>[4x]GPLGSDYIIKEKTVLLQKKDSEGFGFVLRGAKAQTPIEEFTPTPAFPALQYLESVDEGGVAWRAGLRMGDFLIEVNGQNVVKVGHRQVVNMIRQGGNTLMVKVVMVTRHPDM;>[4x]EESTSFQGP

The SHANK (SH3 and multiple ankyrin repeat domain) protein acts as a scaffolding protein located at excitatory glutamatergic synapses; it plays a crucial role in synapse formation, maintenance, function, and development. As one of the key components of SHANK structures, PDZ [Postsynaptic density protein-95(PSD-95)/Discs-large (DLG)/zonula occludens-1(ZO1)] domains are a large class of protein–protein interaction (PPI) modules that are widely conserved from yeast to humans. A canonical PDZ domain is usually composed of roughly 90 amino acid residues, consisting of 5–6 β-strands (βA-βF) capped by a short helix αA and a long α-helix αB, where the N- and C-terminal strands βA and βF are in mutual proximity. Significantly, PDZs possess a highly conserved carboxylate-binding loop formed by the second α-helix (αB) and the second β-strand (βB) in an antiparallel fashion; discoveries and characterization of PBMs have established that C-terminal PBMs predominate.

Here we characterize a short linear motif (SLiM) — EESTSFQGP — as an internal PBM based on its strong binding affinity towards the SHANK1 PDZ domain (SHANK1656–762 hereafter referred to as SHANK1). To obtain further insight into the molecular basis of the SHANK1/Ac-EESTSFQGP-NH2 interaction, the co-crystal structure was solved at a resolution of 1.98 Å. The crystals used for structure determination belonged to the trigonal space group P3221. X-ray crystallographic analyses on the SHANK1/Ac-EESTSFQGP-CONH2 complex identified an asymmetric tetramer with four similar protein-ligand protomers. Overall, the two SHANK1 backbones exhibit extensive overlap with an RSMD of 0.45 Å, with subtle differences within the loops, e.g. Q667-G675PDZ, G680-Q700PDZ, V705-G709PDZ and G748-T748PDZ. Loop flexibility likely contributes to adaptation for binding of the different ligands; comparing the SHANK1/Ac-EESTSFQGP-NH2 and SHANK1/GKAP PBM structures, the loops in the Ac-EESTSFQGP-NH2 bound PDZ appear slightly extended so as to accommodate the N-terminal acetyl group as well as the C-terminal extended motif [Gln (1) — Gly (2) — Pro (3)] of the internal PBM. Crucially, one of the most obvious features of C-terminal PBM recognition is the insertion of the C-terminal carboxylate group of the residue at P0 into the PDZ conserved carboxylate binding loop. Both Phe of the internal ligand and Leu of the C-terminal PBM form hydrogen bonds with three target carboxylate-binding-loop residues, F674PDZ, G675PDZ and F676PDZ, thus contributing significantly to the low-micromolar SHANK1 affinities. Ac-EESTSFQGP-NH2 Glu (-4) and GKAP PBM Ala (-4) interact with Gly680PDZ, whilst the former additionally interacts with Arg736PDZ, which may contribute to the more favourable enthalpic binding for Ac-EESTSFQGP-NH2 compared with GKAP PBM as observed in ITC experiments. Interestingly, Ser(-1) of Ac-EESTSFQGP-NH2 is not involved in interaction and instead Gln (1) compensates by binding to Asp706PDZ — a role fulfilled by Arg(-1) in GKAP PBM.> GSHMSKSLKKLVEESREKNQPEVDMSDRGISNMLDVNGLFTLSHITQLVLSHNKLTMVPPNIAELKNLEVLNFFNNQIEELPTQISSLQKLKHLNLGMNRLNTLPRGFGSLPALEVLDLTYNNLSENSLPGNFFYLTTLRALYLSDNDFEILPPDIGKLTKLQILSLRDNDLISLPKEIGELTQLKELHIQGNRLTVLPPELGNLDLTGQKQVFKAENNPWVTPIADQFQLGVSHVFEYIRSETYKYLYGRHMQANPEPPKKNNDKSKKISRKPLAAKNR

Ras suppressor-1 (Rsu-1) is a leucine-rich repeat (LRR)-containing protein that is crucial for regulating cell adhesion and is involved in such physiological and pathological processes as focal adhesion assembly and tumor metastasis. Rsu-1 interacts with zinc-finger type multi-LIM domain-containing adaptor protein PINCH-1, known to be involved in the integrin-mediated consensus adhesome, but not with its highly homologous family member PINCH-2. Rsu-1 does not have catalytic activity but its primary sequence analysis indicates a leucine-rich repeat (LRR)-containing protein that implicates for protein-binding functions. We also showed that Rsu-1 can be assembled, via PINCH-1-binding, into a heteropentamer complex comprising Rsu-1, PINCH-1, ILK, Parvin, and Kindlin-2, which constitute a major consensus integrin adhesome crucial for focal adhesion assembly.

To gain structural insight into the architecture of Rsu-1, we first crystallized and solved its crystal structure by a single-wavelength anomalous dispersion (SAD) method using a single selenomethionine (SeMet)-substituted crystal. The structure of Rsu-1 was refined at 1.76-Å resolution to an Rwork of 17.3% and an Rfree of 21.7% with good stereochemistry. The structural analysis revealed that Rsu-1 adopts an arc-shaped solenoid architecture with the canonical LRR domain that comprises the N-terminal cap region followed by eight tandem LRRs and the C-terminal cap region with approximate dimensions of 80 Å × 40 Å × 30 Å. The N-terminal cap region consists of one α-helix (residues from 5 to 15) and a loop, whereas the C-terminal cap region of Rsu-1 comprises the ninth β-strand followed by a helix-turn-helix motif. Amphipathic structural features in those N- and C-terminal cap regions shield the hydrophobic core residues in the first and last (eighth) LRRs to stabilize the structural integrity of the LRR domain, respectively. The terminal helix (residues 240–251) in the C-terminal cap region then folds toward the convex surface of the LRR region. A parallel β-sheet with nine β-strands from eight LRR motifs and the following segment composes a characteristic concave surface in the LRR domain of Rsu-1. The structure of Rsu-1 superimposes with that of SDS22 with an RMSD of 1.49 Å for the 195 equivalent Cα atom pairs. Although Rsu-1 comprises two distinct variable sequence lengths (23- and 25-residues) in the LRRs that resemble in part those in the plant-specific (PS) subfamily in the LRR superfamily, our structural analysis strongly suggests that Rsu-1 falls into the SDS22-like subfamily rather than the PS subfamily.>[2x]MTNTDLKPLLDNLRNATEFWNLVKEASATDESTVHNRSYRDALDWLESAALALGDALIAQRKAVGGDHE;> MALVDGFLELERSSGKLEWSAILQKMASDLGFSKILFGLLPKDSQDYENAFIVGNYPAAWREHYDRAGYARVDPTVSHCTQSVLPIFWEPSI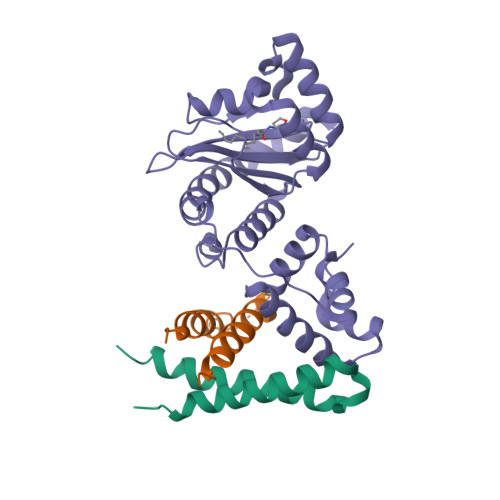YQTRKQHEFFEEASAAGLVYGLTMPLHGARGELGALSLSVEAENRAEANRFMESVLPTLWMLKDYALQSGAGLAFEHPVSKPVVLTSREKEVLQWCAIGKTSWEISVICNCSEANVNFHMGNIRRKFGVTSRRVAAIMAVNLGLITL2-AMINO-ETHANETHIOL | C2 H7 N S | 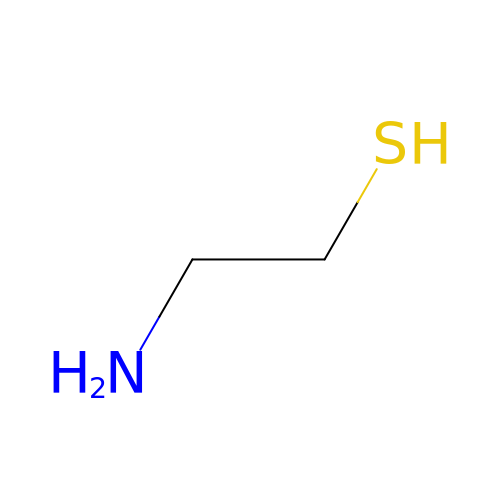UFULAYFCSOUIOV-UHFFFAOYSA-N>[2x]GPHMGSRSRLLAANAAAAAFYAQALQSDEAAPARQYLTERSFDAAAARKFGCGFAPSGWDSLTKHLQRKGFEFEELEAAGLSRQ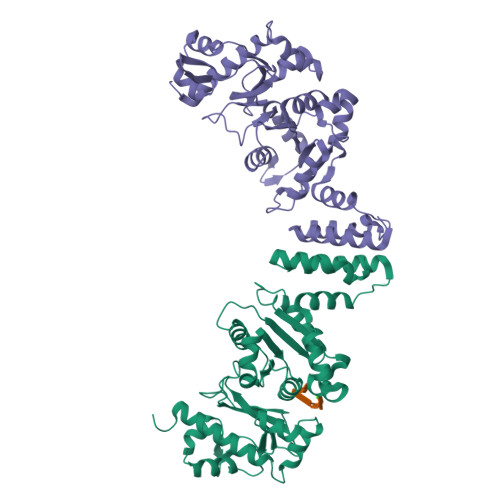GRHGPMDRFHRRLLWPIRTSAGEVVGFGARRLFDDDAMEAKYVNTPETLLYKKSSVMFGIDLAKRDIAKGHQAVVVEGYTDVMAMHLAGVTTAVASCGTAFGGEHLAMLRRLMMDDSFFRGELIYVFDGDEAGRAAALKAFDGEQKLAGQSFVAVAPDGMDPCDLRLKCGDAALRDLVARRTPLFEFAIRAAIAEMDLDSAEGRVAALRRCVPMVGQIKDPTLRDEYARQLAGWVGWADVA> SMYMSNPTVRIAFVGKYLQDAGDTYFSVLQCFEHCQIALQVRLDILYVDSEELEGPNADEARKALLGCDGIFVPGGFGNRGVDGKCAAAQVARMNNIPYFGVCLGMQVAVIELSRNVVGWSDANSEEFNKESTHQVVRIMDCDRNKMGANMHLGACDVYIVEKSSIMAKIYSKSNIVVERHRHRYEVNTAYFEDLRKAGLCISAVTDPTFSSRCRVEAVENPSLRFFLAVQFHPEFISTPMDPAPTYLSFMAAAAKKDYVWPQKCSQRRLKQA

CTP synthetase [EC: 6.3.4.2] catalyzes the formation of CTP from UTP by coupling dephosphorylation of ATP with deamination of glutamine to glutamate, the latter to supply the required amino group. The enzyme, which consists of distinct synthetase and glutaminase domains, is rate limiting in the synthesis of cytosine nucleotides required to maintain RNA and DNA levels. Acivicin, a fermentation product of Streptomyces sviceus, inhibits enzymes like CTP synthetase that catalyze amido transfers from l‐glutamine. The glutaminase domain is dominated by a core β‐sheet of seven strands decorated on one side by six α‐helices, on the other by four helices and two parallel β‐strands.

The glutaminase domain of T. brucei CTP synthetase, (residues 319–589), following incubation with acivicin, crystallized in space group P212121 with one molecule in the asymmetric unit and diffracted to 2.1 Å resolution. We now report an improved and corrected inhibitor structure with changes to the chirality at one position, the orientation and covalent structure of the isoxazoline moiety, and the location of a chloride ion in an oxyanion binding site that is exploited during catalysis. The active site is located at one end of the sheet in a small, ordered, polar cavity. The corrected orientation of the ligand now results in four out of five functional groups participating in hydrogen bonding interactions directly with the enzyme, the fifth to a water molecule that is then in contact with the enzyme. N2 and O3 accept hydrogen bonds donated by the main chain amides of Leu420 and Gly392 respectively. The C1 carboxylate interacts with solvent, and the side chains of basic residues Arg498 and His549. The amino substituent on C2 donates hydrogen bonds to water and the carbonyl of Gly392. The activation of the nucleophilic Cys419 is supported by the position of His549, 3.6 Å distant, which in turn is positioned by a hydrogen bond with the side chain of Glu551. Stabilization of the oxyanion intermediate formed during the reaction with acivicin, or during catalysis may benefit from the position of the amine and amide groups of Gln423, Arg500 and Tyr501 respectively forming a positively charged environment similar to that observed near the cysteine protease‐like catalytic triad in trypanothione synthetase‐amidase. This site is where chloride binds.> KWVMSTKYVEAGELKEGSYVVIDGEPCRVVEIEKSKTGKHGSAKARIVAVGVFDGGKRTLSLPVDAQVEVPIIEKFTAQILSVSGDVIQLMDMRDYKTIEVPMKYVEEEAK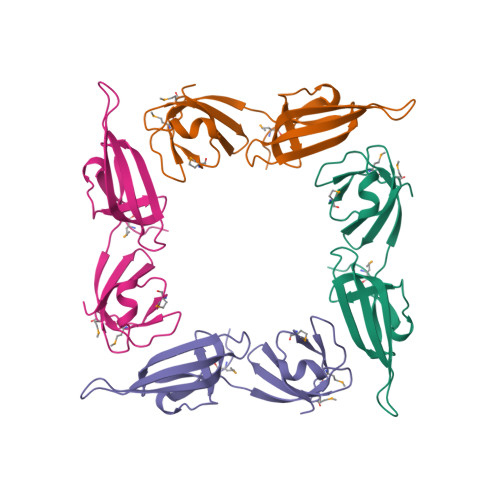GRLAPGAEVEVWQILDRYKIIRVKG> AMITKYLYDENAYDYHDGGYRPLKKAPGEEHPLNVPAFLKPDRIEGNEIYYTVTAQAGETKILPGKPTHTWGYNGSILGPAIQFETGKTYHVTLKNELDEVTTFHWHGLNIVGPYEDGGPHAPVYPHGERKITFTVDQPAANIWLHPHPCPETARQVWNGLAAPVIITDGHEQSLKLPRRWGVNDFPVVLQDRSYHDNQLDYKADYDVDGTLGDYALVNGTVNPVVNVTKPIIRLRFLNGSNRREWRLHFADYHPFTQIGSDGGLLPEAVEMDRIMLTCAERADVLVNFSDYQPGQEVILQTDDFNLIKFKIGD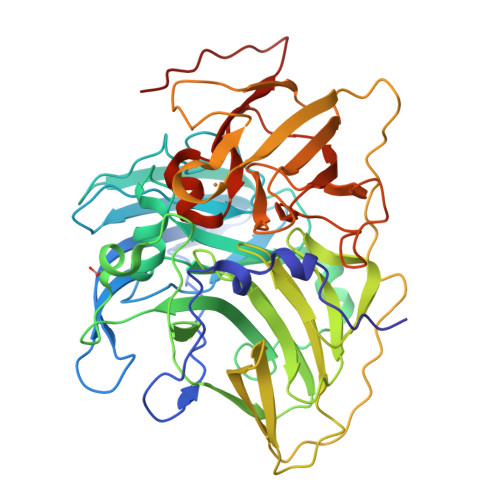IKKENMLLPSPLAEIPALSVDENTPVFKTVMSGMDDQVRLDGKLFDMQRIDTRQQVDQTQIWEVSNTNDMEGGMIHPFHIHGCQFQLIDRNGHAVNPNEHGWKDTIGVNPNETVRIRVKFTKLGIFMYHCHILEHEDTGMMAQIEIFDPDHPIEYHLMPMNHKM6-O-PHOSPHORYL INOSINE MONOPHOSPHATE | C10 H14 N4 O11 P2 | 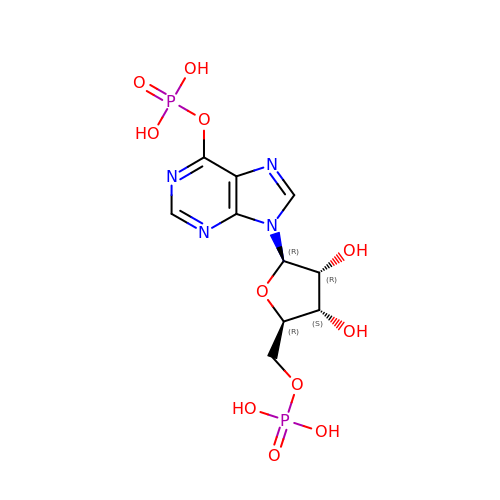RXRZOKQPANIEDW-KQYNXXCUSA-N> MRCIGISNRDFVEGVSGGSWVDIVLEHGSCVTTMAKNKPTLDFELIKTEAKQPATLRKYCIEAKLTNTTTDSRCPTQGEPTLNEEQDKRFVCKHSMVDRGWGNGCGLFGKGGIVTCAMFTCKKNMEGKIVQPENLEYTVVITPHSGEEHAVGNDTGKHGKEVKITPQSSITEAELTGYGTVTMECSPRTGLDFNEMVLLQMKDKAWLVHRQWFLDLPLPWLPGADTQGSNWIQKETLVTFKNPHAKKQDVVVLGSQEGAMHTALTGATEIQMSSGNLLFTGHLKCRLRMDKLQLKGMSYSMCTGKFKVVKEIAETQHGTIVIRVQYEGDGSPCKIPFEIMDLEKRHVLGRLITVNPIVTEKDSPVNIEAEPPFGDSYIII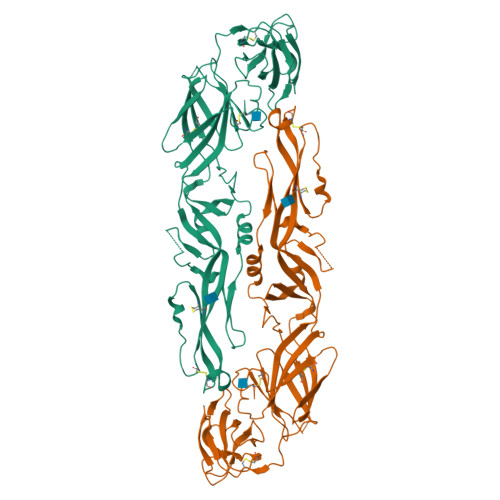GVEPGQLKLDWFKKG> AETVESCLAKSHTENSFTNVWKDDKTLDRYANYEGCLWNATGVVVCTGDETQCYGTWVPIGLAIPENEGGG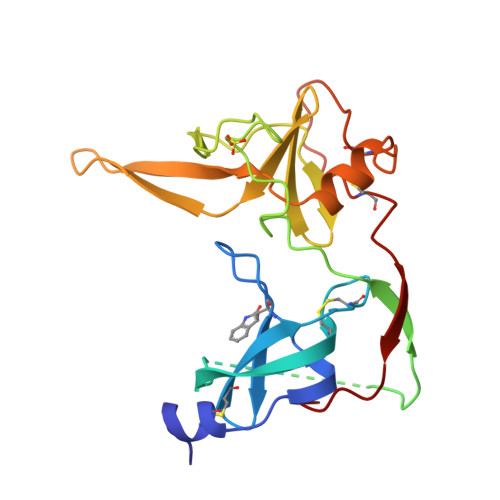SEGGGSEGGGSEGGGTKPPEYGDTPIPGYTYINPLDGTYPPGTEQNPANPNPSLEESQPLNTFMFQNNRFRNRQGALTVYTGTVTQGTDPVKTYYQYTPVSSKAMYDAYWNGKFRDCAFHSGFNEDIFVCEYQGQSSDLPQPPVNA>MHHHHHHSSGRENLYFQGLDVKMDIHVLENFKNYALLLKLQKLAMTIIAQQSNDYDLQQLKTVFLYLDEDGKGNITKNQLKKGLENSGLKLPQNFDVLLDQIDSDGSGRIDYTEFLAAALDRKHLSKKLI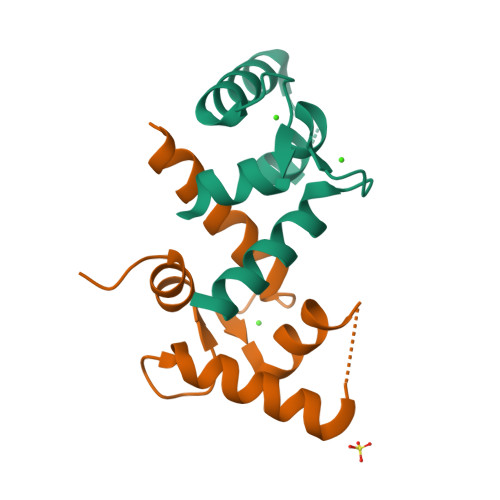YCAFRVFDVDNDGEITTAELAHILYNGNKKGSITQKDVNQVKKMIQEVDKNNDGKIDFYEFCEMMKLKY[2x]> DDLDV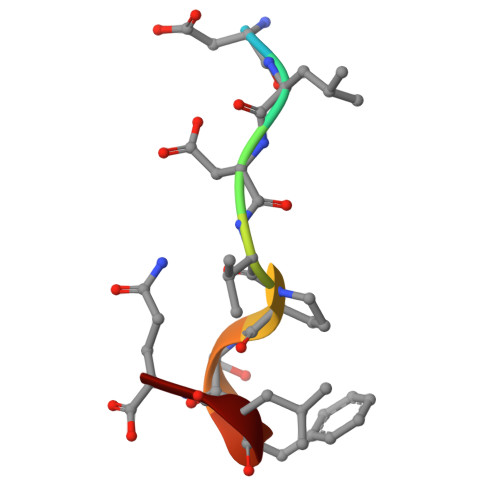PSFLQ>[2x]GSHMNGPIIMTREERMKIVHEIKERILDKYGDDVKAIGVYGSLGRQTDGPYSDIDMMCVMSTEEAEFSHEWTTGEWKVEVNFDSEEILLDYASQVESDWPLTHGQFFSILPIYDSGGYLEKVYQTAKSVEAQKFHDAICALIVEELFEYAGKWRNIRVQGPTTFLPSLTVQVAMAGAMLIGLHHRICYTTSASVLTEAVKQSDLPSGYDHLCQFVMSGQLSDSEKLLESLE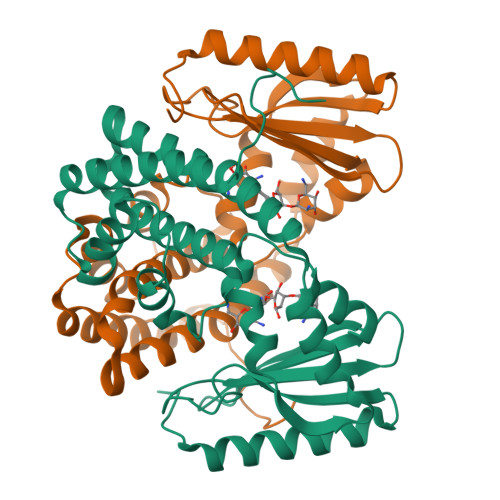NFWNGIQEWTERHGYIVDVSKRIPF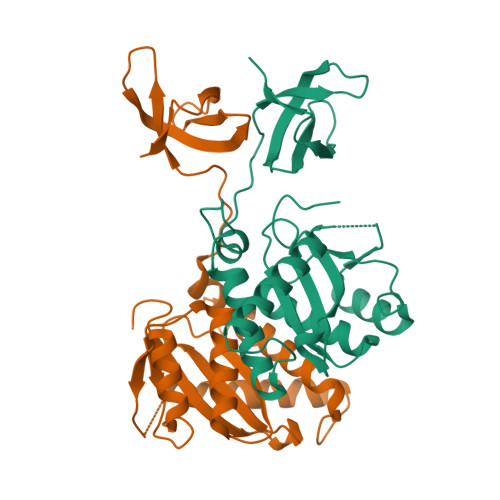>[2x]PLREAKDLHTALHIGPRALSKASNISMQQAREVVQTCPHCNSAPALEAGVNPRGLGPLQIWQTDFTLEPRMAPRSWLAVTVDTASSAIVVTQHGRVTSVAVQHHWATAIAVLGRPKAIKTDNGSCFTSKSTREWLARWGIAHTTGIPGNSQGQAMVERANRLLKDKIRVLAEGDGFMKRIPTSKQGELLAKAMYALNHKERGENTKTPIQKHWRPTVLTEGPPVKIRIETGEWEKGWNVLVWGRGYAAVKNRDTDKVIWVPSRKVKPDIT>[2x]GAGUAG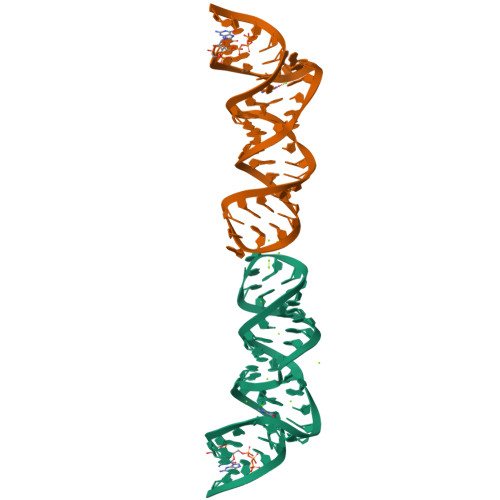AAGCGUUCAGCGGCCGAAAGGCCGCCCGGAAAUUGCUCC>MKYQLTALEARVIGCLLEKQVTTPEQYPLSVNGVVTACNQKTNREPVMNLSESEVQEQLDNLVKRHYLRTVSGFGNRVTKYEQRFCNSEFGDLKLSAAEVALITTLLLRGAQTPGELRSRAARMYEFSDMAEVELTLEQLANREDGPFVVRLAREPGKRESRYMHLFSGEVEDQPAVTDMSN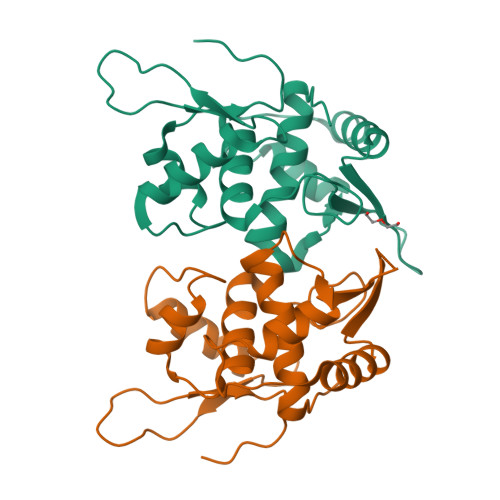AVDGDLQARVEALEIEVAELKQRLDSLLAHLGD[2x]> CTEPLGLKDNTIPNKQITASSYYKTWGLSAFSWFPYYARLDNQGKFNAWTAQTNSASEWLQIDLGSQKRVTGIITQGARDFGHIQYVAAYRVAYGDDGVTWTEYKDPGASESKIFPGNMDNN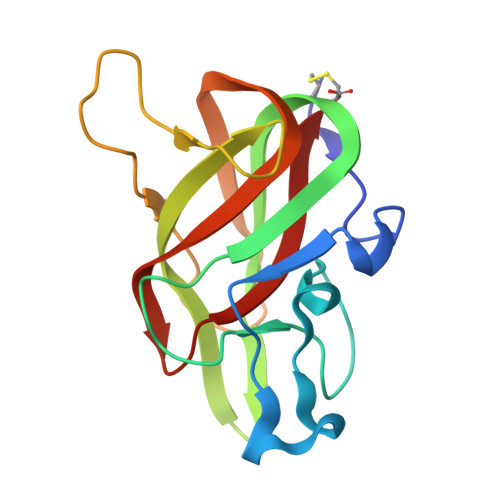SHKKNIFETPFQARFVRIQPVAWHNRITLRVELLGC4-[(6-CHLORO-2-NAPHTHALENYL)SULFONYL]-1-[[4-HYDROXYIMINOMETHYL-1-(4-PYRIDINYL)-4-PIPERIDINYL]METHYL]PIPERAZINONE 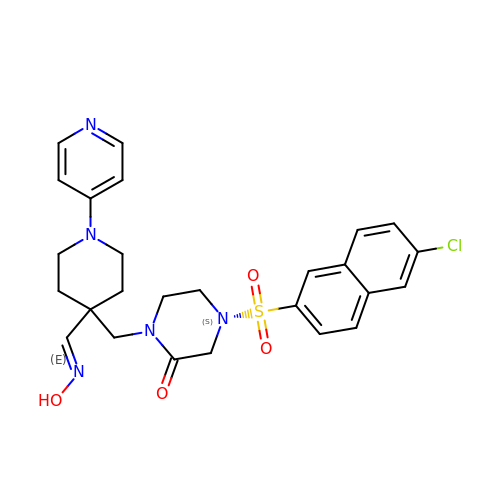| C26 H28 Cl N5 O4 S | UELXXBOTHARRQL-RDRPBHBLSA-N> NPYNIVPQGRIVSLTNA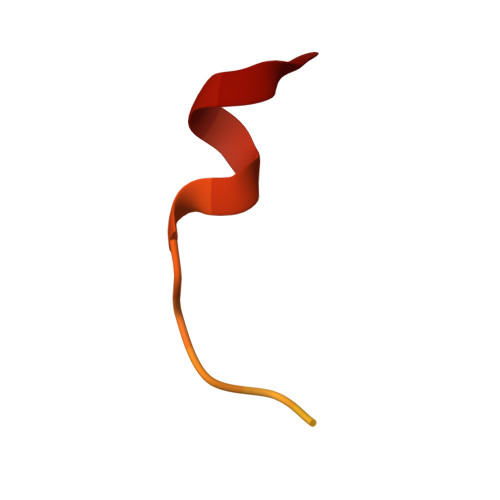QNRERLQLLEE>G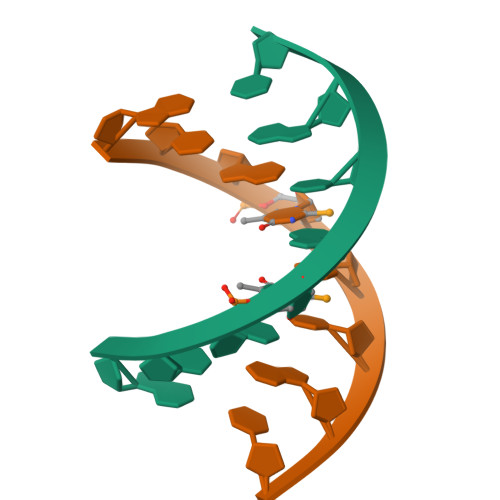TGTACAC[2x]>[4x]MGKRMVVVGGVAGGASAAAKAKRENPELEVVVYEKSGWVSYGACGLPYVLSGEIPRLERLVARTPEEFRKQGVLVHTRHEVVDVDYELRTLTVHDHAEGRTFQDRFDHLVLATGARPSLPPIPGTEQEGVYTLRTMEDGERLL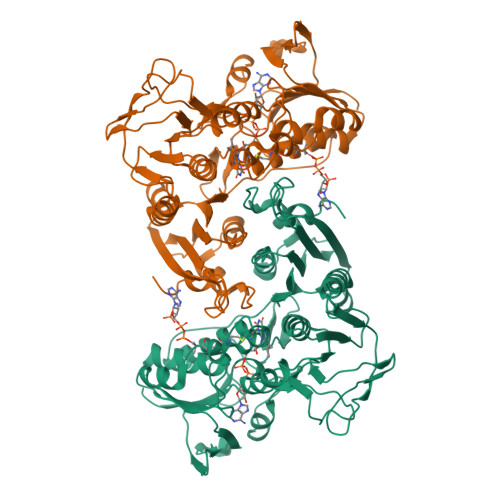KALPQARRAAILGAGYIGLEAAEAFRKRGLQVTLLEAKDRPLPHWDPEVGALLKEELERHGVEVWTGVKVEAFRGMGRVEAVETSEGVVPADLVLLATGIRPNTELAQAMGVALGPTGAIATDERMRTNLEGVYAAGDVAESFHRVLKRPYWLPLGDVANKHGRTAGSVIAGREARFLGVVGTAIFKAFDLAVATTGLSLEGALKEGFWAKKVFIQSRDGAHYYPGSGPLWVELVYEEGTGRLLGGAVVARGHGALRIDVLAALLHREGSVEDLLALDLAYAPPFSPVWDPLLIAAQQAR> MSIKPGTYEVTSKVNGLHVGRPLAEDRSLLPKRIRVLPEDNNSGNSWVVEKDDDAYILYCKGAPVAPQ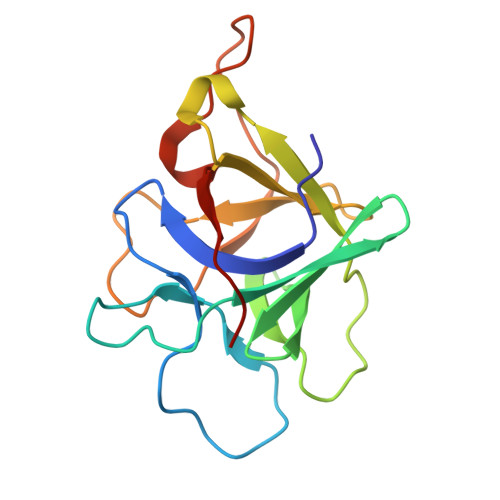EGKLFADLLGNMEDKKWIVTHQPQHGENVFTVVNASTEHGWVVPADAEELQQVEVRPLIAAPSYPPRYPATELFTFTQVESD(2S,3S,4R,5S)-2-(4-methoxyphenyl)-5-methylpyrrolidine-3,4-diol 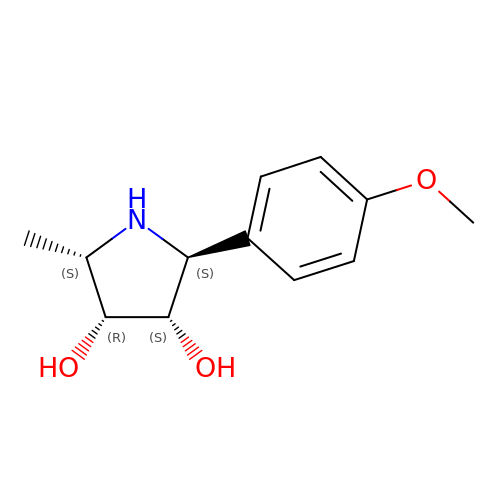| C12 H17 N O3 | RMKWLQBEDHKISQ-VKZDFBPFSA-N> MAGVKNSIIWFRKGLRLHDNPALLEACKDAKHVYPVFVLDPHFLQQSSYKVSVNRYNFLLESLEDLQRSFQARGSRLLVLRGKPEEVFPRVFREWGVTQLCFEHDTEPYAKVRDAAVRRLAAEAGVEVVTPISHTLYDTDMLVARNGGAAPLTMQSFTKLVDRVGDPPAPAPDPPAAMPPPAEDMPSAAPAATGVPTWQEVGFKEPPLTVFKGGETEALARLEAAFQDPKWVAGFQKPDTDPSAWEKPATTVLSPYLKFGCLSARLFHARLLEVYRRHPAHSQPPVSLRGQLLWREFFYTVGSTTPNFHRMAGNPVCKQIDWDDNPEFLAAWREARTGFPWIDAIMTQLVTW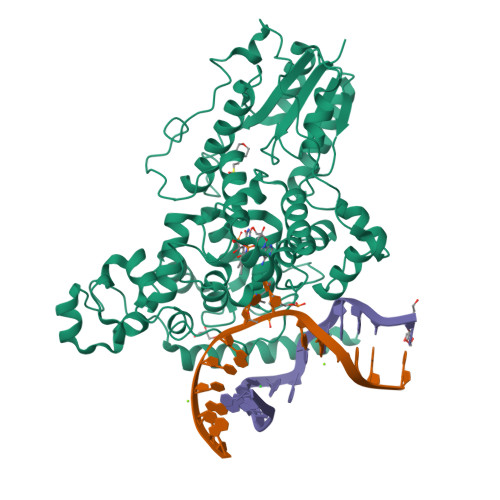GWMHHLARHSVACFLTRGDLYVSWERGMEVFEEHLIDQDHYLNAANWMWLSASAFFSQYFRVYSPVVFGKKYDPEGRFIRKFLPVLKDMPAKYIYEPWTAPLEVQRKAGCVVGRDYPAPIVDHAVASKACIARMAAAYRRSKGEKLA> FSEEEVRYEIIL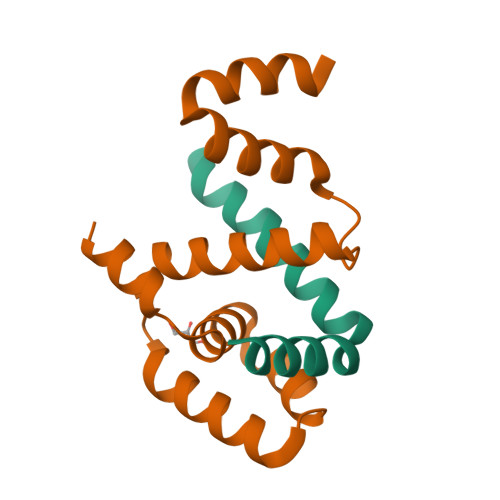EKIRGTLKERPDEIAMLFKLLIKDE;> PKQKAQLDELSMSEKIAILLIQVGEDTTGEILRHLDIDSITEISKQIVQLNGTDKQIGAAVLEEFFAIFQSNQYINTGGLEYARELLTRTLGSEEAKKVMDKLTK> MSRFVTSVSALAMLALAPAALSSGAYANDKLVELSKSDDNWVMPGKNYDSNNFSDLKQINKGNVKQLRPAWTFSTGLLNGHEGAPLVVDGKMYIHTSFPNNTFALGLDDPGTILWQDKPKQNPAARAVACCDLVNRGLAYWPGDGKTPALILKTQLDGNVAALNAETGETVWKVEN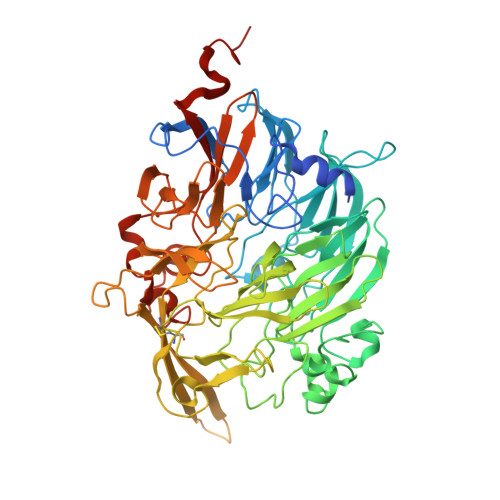SDIKVGSTLTIAPYVVKDKVIIGSSGAELGVRGYLTAYDVKTGEQVWRAYATGPDKDLLLASDFNIKNPHYGQKGLGTGTWEGDAWKIGGGTNWGWYAYDPGTNLIYFGTGNPAPWNETMRPGDNKWTMTIFGRDADTGEAKFGYQKTPHDEWDYAGVNVMMLSEQKDKDGKARKLLTHPDRNGIVYTLDRTDGALVSANKLDDTVNVFKSVDLKTGQPVRDPEYGTRMDHLAKDICPSAMGYHNQGHDSYDPKRELFFMGINHICMDWEPFMLPYRAGQFFVGATLNMYPGPKGDRQNYEGLGQIKAYNAITGDYKWEKMERFAVWGGTMATAGDLVFYGTLDGYLKARDSDTGDLLWKFKIPSGAIGYPMTYTHKGTQYVAIYYGVGGWPGVGLVFDLADPTAGLGAVGAFKKLANYTQMGGGVVVFSLDGKGPYDDPNVGEWKSAAKHHHHHH> MSDAAPSLSNLFYDPTYNPGQSTINYTSIYGNGSTITFDELQGLVNSTVTQAIMFGVRCGAAALTLIVMWMTSRSRKTPIFIINQVSLFLIILHSALYFKYLLSNYSSVTYALTGFPQFISRGDVHVYGATNIIQVLLVASIETSLVFQIKVIFTGDNFKRIGLMLTSISFTLGIATVTMYFVSAVKGMIVTYNDVSATQDKYFNASTILLASSINFMSFVLVVKLILAIRSRRFLGLKQFDSFHILLIMSCQSLLVPSIIFILAYSLKPNQGTDVLTTVATLLAVLSLPLSSMWATAANNASKTNTITSDFTTSTDRFYPGTLSSFQTDSINNDAKSSLRSRLYDLYPRRKETTSDKHSERTFVSETADDIEKNQFYQLPTPTSSKNT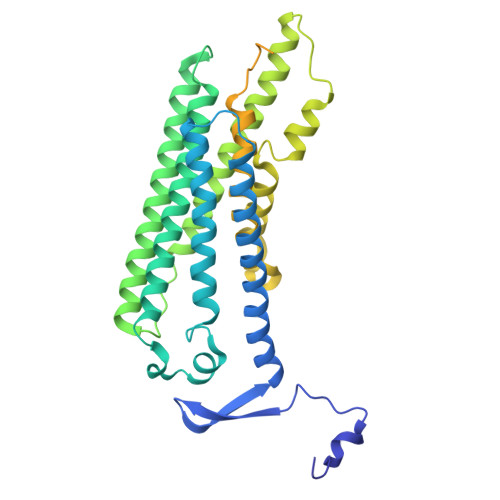RIGPFADASYKEGEVEPVDMYTPDTAADEEARKFWTEDNNNL Respiratory complex I is a multi-subunit membrane protein complex that reversibly couples NADH oxidation and ubiquinone reduction with proton translocation against transmembrane potential. Complex I from all characterized species contains homologues of 14 core subunits; seven subunits each assemble into peripheral and membrane arms, joined at their tips and form the complex with a characteristic L-shape. The peripheral arm, exposed to the cytoplasm in bacteria or the mitochondrial matrix in eukaryotes, contains binding sites for NADH, ubiquinone, and flavin mononucleotide (FMN) as well as eight or nine iron-sulfur clusters, seven of which connect the NADH and ubiquinone-binding sites enabling rapid electron transfer. Here, we describe the single particle cryo-electron microscopy (cryo-EM) structure of the entire catalytically active E. coli complex I reconstituted into lipid nanodiscs.

After density modification, the resolution of membrane arm improved to 3.7 Å. The model of complete membrane arm, including the previously missing subunit NuoH, was built into the density map with local resolution better than 3.5 Å at the arm center and approximately 4.0 Å at its periphery. An additional density belt corresponding to the lipid nanodisc is clearly visible around the membrane-embedded region. The structure of the membrane arm in the lipid nanodisc is very similar to the crystal structure of the detergent-solubilized membrane arm [RMSD of 1.1 Å (1888 Cα)]. The density for the N-terminus of NuoH (residues 1–52) that includes HTMH1 and a part of HTMH1-TMH2 loop, is completely missing in the reconstructions of the membrane fragment and of the complete complex. The structures visualize a complete chain of charged residues connecting the Q-site with charged residues in antiporter-like subunits. Thus, analysis of the protein translocation pathways indicates that in E. coli, no continuous proton path exists between the Q-site and NuoN. The density of the cytoplasmic half of MTM8 is poor and fragmented between residues 255 and 265, indicating the existence of multiple conformations. Conversely, MTMH8 displays localized disorder next to the π-bulge, indicating possible involvement of this helix in the structural rearrangements associated with proton translocation, and to our knowledge, this represents the first indication of specific conformational changes in antiporter-like subunits.

> MSMSTSTEVIAHHWAFAIFLIVAIGLCCLMLVGGWFLGGRARARSKNVPFESGIDSVGSARLRLSAKFYLVAMFFVIFDVEALYLFAWSTSIRESGWVGFVEAAIFIFVLLAGLVYLVRIGALDWTPARSRRERMNPETNSIANRQR;> MSWISPELIEILLTILKAVVILLVVVTCGAFMSFGERRLLGLFQNRYGPNRVGWGGSLQLVADMIKMFFKEDWIPKFSDRVIFTLAPMIAFTSLLLAFAIVPVSPGWVVADLNIGILFFLMMAGLAVYAVLFAGWSSNNKYSLLGAMRASAQTLSYEVFLGLSLMGVVAQAGSFNMTDIVNSQAHVWNVIPQFFGFITFAIAGVAVCHRHPFDQPEAEQELADGYHIEYSGMKFGLFFVGEYIGIVTISALMVTLFFGGWQGPLLPPFIWFALKTAFFMMMFILIRASLPRPRYDQVMSFGWKICLPLTLINLLVTAAVILWQAQ;> MEFAFYICGLIAILATLRVITHTNPVHALLYLIISLLAISGVFFSLGAYFAGALEIIVYAGAIMVLFVFVVMMLNLGGSEIEQERQWLKPQVWIGPAILSAIMLVVIVYAILGVNDQGIDGTPISAKAVGITLFGPYVLAVELASMLLLAGLVVAFHVGREERAGEVLSNRKDDSAKRKTEEHA;> MIPLQHGLILAAILFVLGLTGLVIRRNLLFMLIGLEIMINASALAFVVAGSYWGQTDGQVMYILAISLAAAEASIGLALLLQLHRRRQNLNIDSVSEMRG;> MNMLALTIILPLIGFVLLAFSRGRWSENVSAIVGVGSVGLAALVTAFIGVDFFANGEQTYSQPLWTWMSVGDFNIGFNLVLDGLSLTMLSVVTGVGFLIHMYASWYMRGEEGYSRFFAYTNLFIASMVVLVLADNLLLMYLGWEGVGLCSYLLIGFYYTDPKNGAAAMKAFVVTRVGDVFLAFALFILYNELGTLNFREMVELAPAHFADGNNMLMWATLMLLGGAVGKSAQLPLQTWLADAMAGPTPVSALIHAATMVTAGVYLIARTHGLFLMTPEVLHLVGIVGAVTLLLAGFAALVQTDIKRVLAYSTMSQIGYMFLALGVQAWDAAIFHLMTHAFFKALLFLASGSVILACHHEQNIFKMGGLRKSIPLVYLCFLVGGAALSALPLVTAGFFSKDEILAGAMANGHINLMVAGLVGAFMTSLYTFRMIFIVFHGKEQIHAHAVKGVTHSLPLIVLLILSTFVGALIVPPLQGVLPQTTELAHGSMLTLEITSGVVAVVGILLAAWLWLGKRTLVTSIANSAPGRLLSTWWYNAWGFDWLYDKVFVKPFLGIAWLLKRDPLNSMMNIPAVLSRFAGKGLLLSENGYLRWYVASMSIGAVVVLALLMVLR;> MLLPWLILIPFIGGFLCWQTERFGVKVPRWIALITMGLTLALSLQLWLQGGYSLTQSAGIPQWQSEFDMPWIPRFGISIHLAIDGLSLLMVVLTGLLGVLAVLCSWKEIEKYQGFFHLNLMWILGGVIGVFLAIDMFLFFFFWEMMLVPMYFLIALWGHKASDGKTRITAATKFFIYTQASGLVMLIAILALVFVHYNATGVWTFNYEELLNTPMSSGVEYLLMLGFFIAFAVKMPVVPLHGWLPDAHSQAPTAGSVDLAGILLKTAAYGLLRFSLPLFPNASAEFAPIAMWLGVIGIFYGAWMAFAQTDIKRLIAYTSVSHMGFVLIAIYTGSQLAYQGAVIQMIAHGLSAAGLFILCGQLYERIHTRDMRMMGGLWSKMKWLPALSLFFAVATLGMPGTGNFVGEFMILFGSFQVVPVITVISTFGLVFASVYSLAMLHRAYFGKAKSQIASQELPGMSLRELFMILLLVVLLVLLGFYPQPILDTSHSAIGNIQQWFVNSVTTTRP;> MTITPQNLIALLPLLIVGLTVVVVMLSIAWRRNHFLNATLSVIGLNAALVSLWFVGQAGAMDVTPLMRVDGFAMLYTGLVLLASLATCTFAYPWLEGYNDNKDEFYLLVLIAALGGILLANANHLASLFLGIELISLPLFGLVGYAFRQKRSLEASIKYTILSAAASSFLLFGMALVYAQSGDLSFVALGKNLGDGMLNEPLLLAGFGLMIVGLGFKLSLVPFHLWTPDVYQGAPAPVSTFLATASKIAIFGVVMRLFLYAPVGDSEAIRVVLAIIAFASIIFGNLMALSQTNIKRLLGYSSISHLGYLLVALIALQTGEMSMEAVGVYLAGYLFSSLGAFGVVSLMSSPYRGPDADSLFSYRGLFWHRPILAAVMTVMMLSLAGIPMTLGFIGKFYVLAVGVQAHLWWLVGAVVVGSAIGLYYYLRVAVSLYLHAPEQPGRDAPSNWQYSAGGIVVLISALLVLVLGVWPQPLISIVRLAMPLM>MSDYKDDDDKGGGGSMAIAHLATEYVFSDFLLKEPTEPKFKGLRLELAVDKMVTCIAVGLPLLLISLAFAQEISIGTQISCFSPSSFSWRQAAFVDSYCWAAVQQKSSLQSESGNLPLWLHKFFPYILLLFAILLYLPALFWRFSAAPHLCSDLKFIMEELDKVYNRAIKAAKSARDLDLRDGPGPPGVTENVGQSLWEISESHFKYPIVEQYLKTKKNSSHLIMKYISCRLVTFVVILLACIYLSYYFSLSSLSDEFLCSIKSGVLK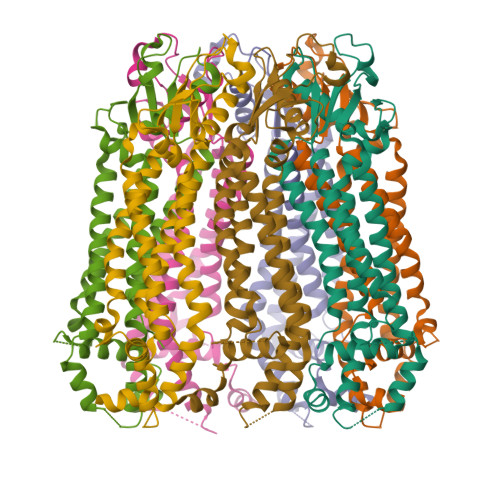NDSTIPDRFQCKLIAVGIFQLLSLINLIVYALLIPVVVYTFFIPFRQKTDILKVYEILPTFDVLHFKSEGYNDLSLYNLFLEENISELKSYKCLKVLENIKSNGQGIDPMLLLTNLGMIKMDIIDGKIPTSLQTKGEDQGSQRVEFKDLDLSSEAAANNGEKNSRQRLLNPSCLEVLFQ[7x]> 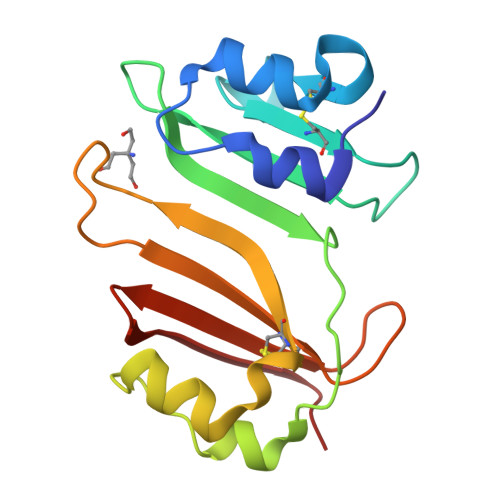SGFSAEKYEQIQFGMTFDEVWEIGGGEAACDTGGVIGDSILCFTESGDYAPYGGFSFTDEGELWSKRNEYLYKAKTPSVKLSHYNRTALGMTEAQLWAAVPKDSCVSQGESYPNWPAKTGFEEKYYCAAATGLFPPSASFHLTDGVLTYRYQRSLT>MSGAPPPSSGFAPRSYGQQPLSHAPRSSMMSVEYDGIPLPPPSIRSCGSQQYVTSYIPTGAAFPPSSVQDMISSMKSYASATDLVRTYSEIPSVEEALSTLDRAAAALNARRYRDALKLYLEGGYAMANVAERQANPKICNLLTSKGFETLNWCARLCDWIEGRIKEKHPRPGVHKVGIPVSNWDEDWVGPFMDEEEARRMWYTPVYCPHPIDFSNLGYRLRCVETGRRPRLMICITMYNEGPQQLKATLKKLANNLAYLKEQMPGDEKSLTGAFAGDDVWQNVLVCIVADGREQVHPKTLDYLEAIGLYDEDLLTINSAGIGAQCHLFEHTLQLSVNGKCLLPIQTVFALKENKASKLDSHHWYFNAFAEQIQPEYTAVMDVGTMLTKSALYHLLFAFERNHQIGGACGQLTVDNPFENLSNWVISAQHFEYKISNILDKSLESCFGFISVLPGAFSAYRYEAIRGAPLDAYFQTLNIELDVLGPFIGNMYLAEDRILSFEVVARKNCNWTMHYVKDAVARTDVPHDLVGLISQRKRWLNGAFFATLFSIWNWGRIYSESKHTFVRKMAFLVFYVYHLLYTAFGFFLPANLYLALFFIVFQG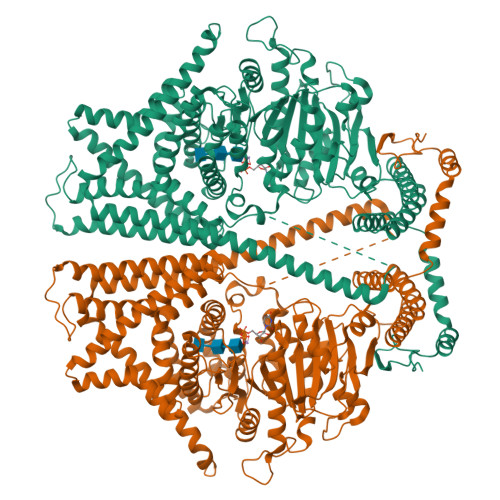FQQNRLEFIDTSEYSQTVLDCAVYIYNFSYLFGLLMLIIIGLGNNPKHMKLTYYFVGAVFGLMMMLSSLVGAGIFFSTPATVHSIVVSILTVGVYFIASALHGEVHHIFMTFTHYTALIPSFVNIFTIYSFCNLQDLSWGTKGLHDDPLLAASLDETEKGDFKDVIAKRRALEELRREEKERVENRKKNFEAFRTNVLLTWAFSNLIFALFVVYFASSSTYMPVLYIFVASLNTCRLLGSIGHWVYIHTEGLRGRVIDKSECGNGTGRYPQNSYVQLEEHYAALAEDQRTYASGRTNASVRTVNDVSSAA[2x]> MVTAHTNHGDIVIKTFDDKAPETV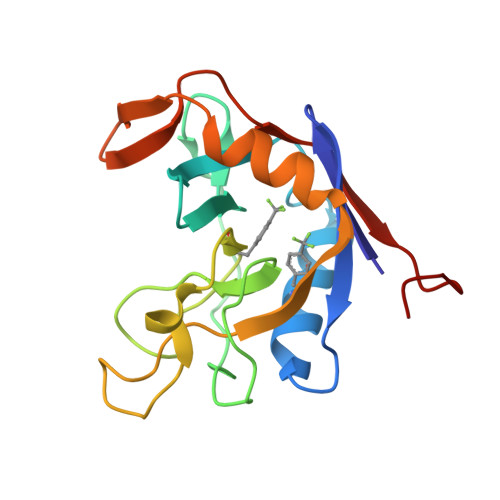KNFLDYCREGFYNNTIFHRVINGFMIQGGGFEPGMKQKATKEPIKNEANNGLKNTRGTLAMARTQAPHSATAQFFINVVDNDFLNFSGESLQGWGYCVFAEVVDGMDVVDKIKGVATGRSGMHQDVPKEDVIIESVTVSEHHHHHH>MDYILGRYVKIARYGSGGLVGGGGKEQYVENLVLWENIIKTAYCFITPSSYTAALETANIPEKDFSNCFRFLKENFFIIPSEYNNSTENNRYSRNFLHYQSYGANPVLVQDKLKNAKVVILGCGGIGNHVSVILATSGIGEIILIDNDQIENTNLTRQVLFS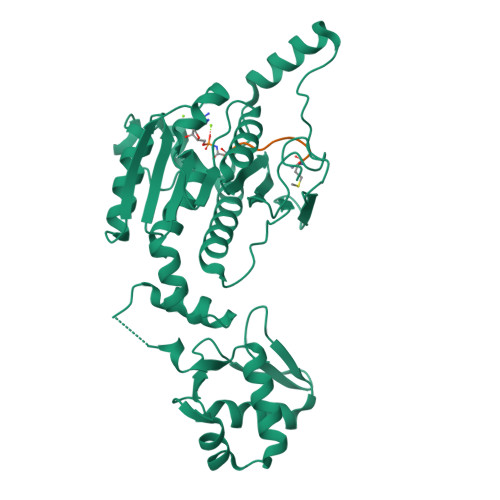EDDVGKNKTEVIKRELLKRNSEISVSEIALNINDYTDLHKVPEADIWVVSADHPFNLINWVNKYCVRANQPYINAGYVNDIAVFGPLYVPGKTGCYECQKVVADLYGAEKENIDHKIKLINSRFKPATFAPVNNVAAALCAADVIKFIGKYSEPLSLNKRIGIWSDEIKIHSQNMGRSPVCSVCGN[2x];>MRTGNAD[2x]> GPLGSMSWGTELWDQFDNLEKHTQWGIDILEKYIKFVKERTEIELSYAKQLRNLSKKYQPKKNSKEEEEYKYTSCKAFISNLNEMNDYAGQHEVISENMASQIIVDLARYVQELKQERKSNFHDGRKAQQHIETCWKQLESSKRRFERDCKEADRAQQYFEKMDADINVTKADVEKARQQAQIRHQMAEDSKADYSSILQKFNHEQHEYYHTHIPNIFQKIQEMEERRIVRMGESMKTYAEVDRQVIPIIGKCLDGIVKAAESIDQK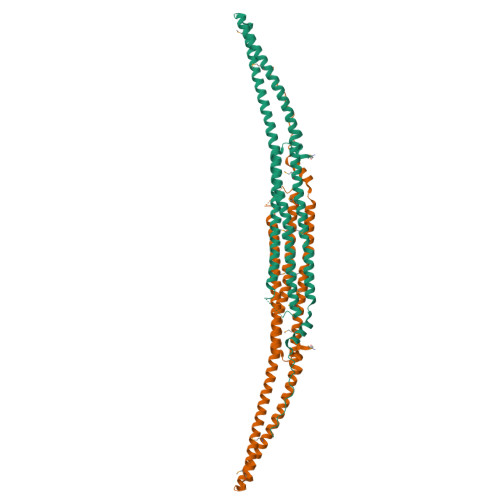NDSQLVIEAYKSGFEPPGDIEFEDYTQPMKRTVSDNSL> MSHYDILQAPVISEKAYSAMERGVYSFWVSPKATKTEIKDAIQQAFGVRVIGISTMNVPGKRKRVGRFIGQRNDRKKAIVRLAE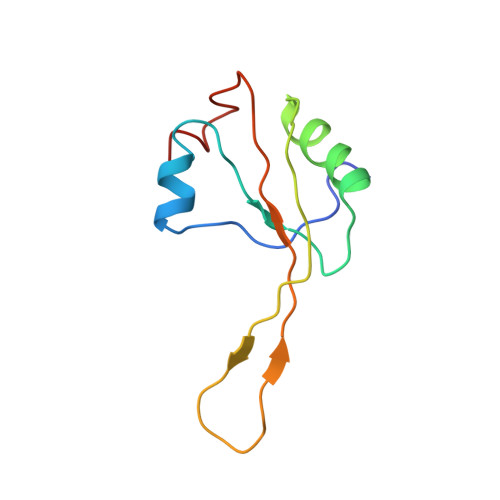GQSIEALAGQA> MSSKYAVKLKTDFDNPRWIKRHKHMFDFLDINGNGKITLDEIV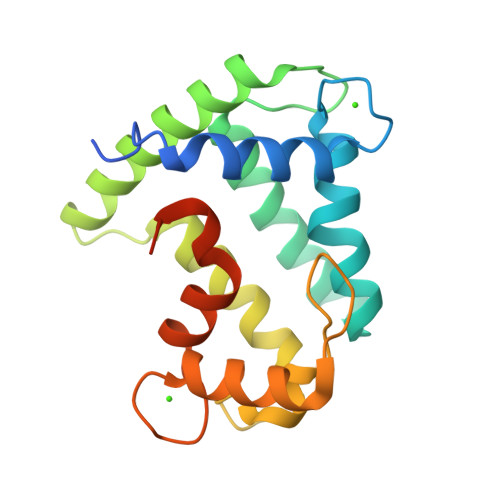SKASDDICAKLEATPEQTKRHQVCVEAFFRGCGMEYGKEIAFPQFLDGWKQLATSELKKWARNEPTLIREWGDAVFDIFDKDGSGTITLDEWKAYGKISGISPSQEDCEATFRHCDLDDSGDLDVDEMTRQHLGFWYTLDPEADGLYGNGVP> GAMGSVNIPRKEKDFQGMLEYKKEDEQKLVKNLILELKPRGVAVNLIPGLPAYILFMCVRHADYLNDDQKVRSLLTSTINSIKKVLKKRGDDFETVSFWLSNTCRFLHCLKQYSGEEGFMKHNTSRQNEHCLTNFDLAEYRQVLSDLAIQIYQQLVRVLENILQPMIVSGMLEHETIQGVSGVKPTGLRKRTSSIADEGTYTLDSILRQLNSFHSVMCQHGMDPELIKQVVKQMFYIIGAITLNNLLLRKDMCSWSKGMQIRYNVSQLEEWLRDKNLMNSGAKETLEPLIQAAQLLQVK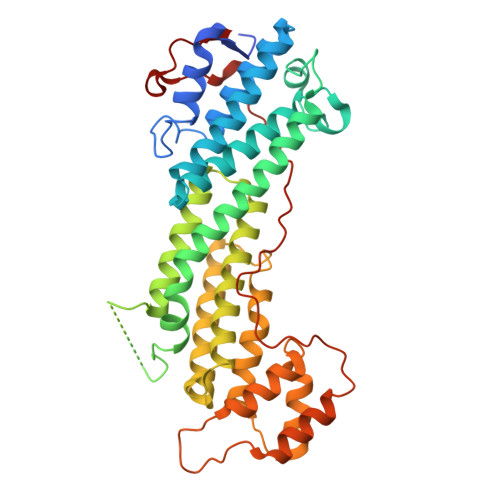KKTDDDAEAICSMCNALTTAQIVKVLNLYTPVNEFEERVSVSFIRTIQMRLRDRKDSPQLLMDAKHIFPVTFPFNPSSLALETIQIPASLGLGFISRV> MSEPEVPFKVVAQFPYKSDYEDDLNFEKDQEIIV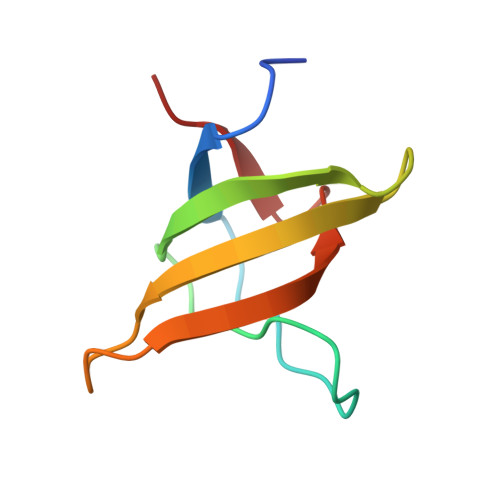TSVEDAEWYFGEYQDSNGDVIEGIFPKSFVAVQG HYDROXY[3-(6-METHYLPYRIDIN-2-YL)PROPYL]FORMAMIDE | C10 H14 N2 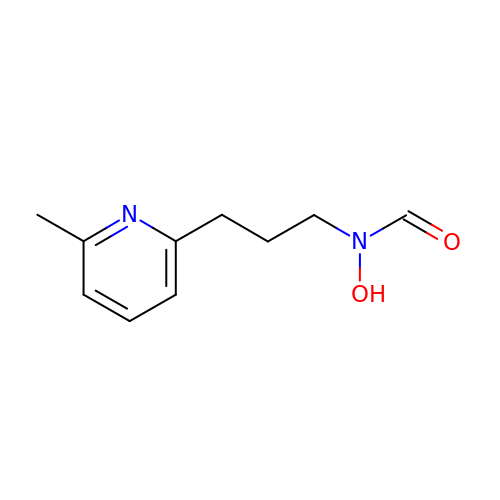O2 | FJYUGRZKJXCRFF-UHFFFAOYSA-N>GIHLGELGLLPSTVLAIGYFENLVNIICESLNMLPKLEVSGKEYKKFKFTIVIPKDLDANIKKRAKIYFKQKSLIEIEIPTSS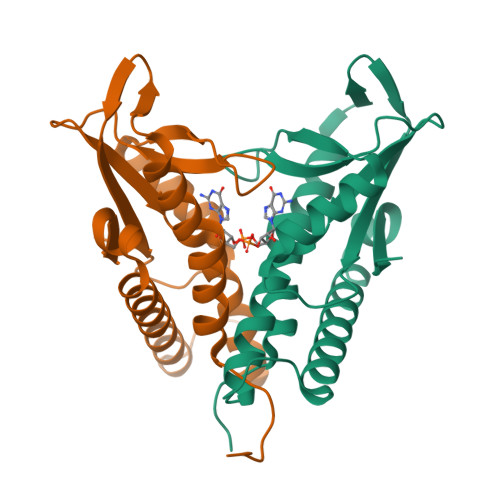RNYPIHIQFDENSTDDILHLYDMPTTIGGIDKAIEMFMRKGHIGKTDQQKLLEERELRNFKTTLENLIATDAFAKEMVEVIIEE[2x]3-(4-IODO-PHENYL)-2-MERCAPTO-PROPIONIC ACID | C9 H9 I O2 S | 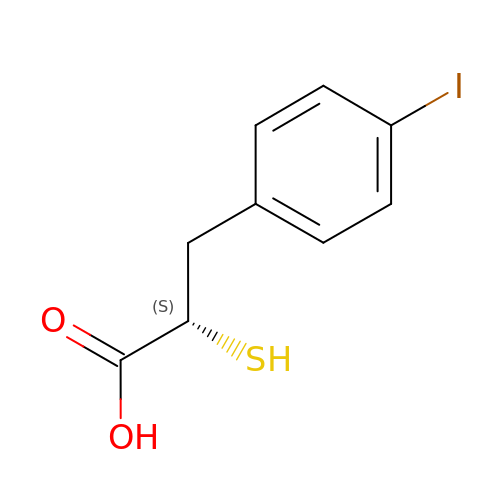MXQYDIIKDPMYMF-QMMMGPOBSA-N> SNAASDLYPLPAPIIDVFPDDGLAKDMAKNLNKDSVNDVIDQDDLDALTGLGFETSTITNDSMQLLERAMFNNVTDVSIMEFGAKLTEFPDITTIPHLKTLFFADPPGRLTRNLSLPNYQNYPEMDTITMSGNNLIGSIPDFTGMPALKQLYMSEMLITSDELPNFNNIPLLITLDLSSNQLTTIPDFQNIPNLTFLDLNANLLTNTPDFQNLPKLTDLNLRHNNLTGTMVNYTNLPSLESLNLDYNFLTELPSNVLDTIYVQSQNGELPDQTINQGDTCTIDLPIYFQMEETNMLVSPEVTGEYIGISVIQLPTTVNEEGNTITVDTSALSPGEYKLDVSYNHNYATGGVCSYDW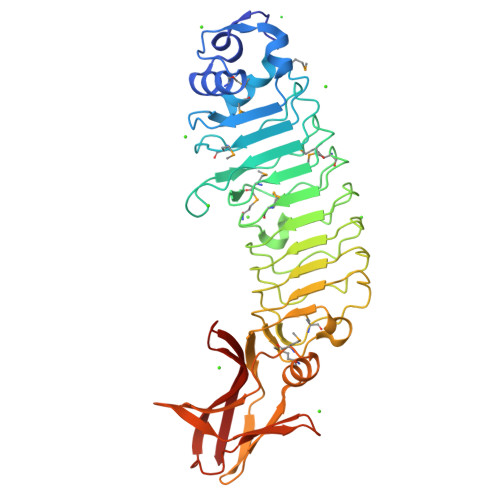NVTIN Twisted gastrulation (TWSG1) is an evolutionarily conserved secreted glycoprotein which controls signaling by Bone Morphogenetic Proteins (BMPs). TWSG1 binds BMPs and their antagonist Chordin to control BMP signaling during embryonic development, kidney regeneration and cancer. TWSG1 is composed of two distinct, disulfide-rich domains. The TWSG1 N-terminal domain occupies the BMP type 1 receptor binding site on BMPs, whereas the C-terminal domain binds to a Chordin family member.

Serendipitously, the TWSG1–GDF5 complex crystallized in the presence of CaCl2, and we identified a calcium-binding site that mediated TWSG1–GDF5 interactions at the periphery of the binding interface. Unexpectedly, the structure of the TWSG1–GDF5 complex reveals a previously unknown calcium-binding site at the edge of TWSG1–GDF5 interface. We confirmed the identity of the calcium ions by anomalous difference Fourier analysis. The calcium ion is coordinated by 8 oxygen atoms with an average distance of 2.55 Å: carboxyl group of GDF5 Asp416, main-chain carbonyl oxygen of GDF5 Gly413 and 5 water molecules. 2 out of 5 water molecules bridge the calcium ion to the carboxyl group of TWSG1 Asp34. The calcium-binding site is stabilized by a hydrogen bond between TWSG1 Ser33 and GDF5 Trp414, and other interactions (salt bridge between TWSG1 Asp34 and Lys37; T-shaped π-π stacking of Trp414 and Trp417 of GDF5). The mutation of the calcium-binding residue Asp34 to Ala in TWSG1 did not abolish the TWSG1–BMP interactions, indicating a minor regulatory role for calcium. Since the calcium-binding residues in BMP ligands are conserved, and calcium is ubiquitously present in the extracellular space, our TWSG1–GDF5 structure brings this ion into focus.

>[2x]MAPLATRQGKRPSKNLKARCSRKALHVNFKDMGWDDWIIAPLEYEAFHCEGLCEFPLRSHLEPTNHAVIQTLMNSMDPESTPPTCCVPTRLSPISILFIDSANNVVYKQYEDMVVESCGCR;>ETGCNKALCASDVSKCLIQELCQCRPGEGNCSCCKECMLCLGALWDECCDCVGMCNPRNYSGTLEVLFQ[2x]>[4x]MSTLEQTIGNTPLVKLQRMGP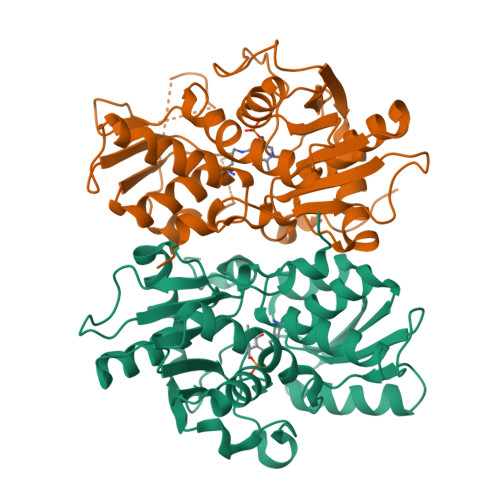DNGSEVWLKLEGNNPAGSVKDRAALSMIVEAEKRGRIKPGDVLIEATSGNTGIALAMIAALKGYRMKLLMPDNMSQERRAAMRAYGAELILVTKEQGMEGARDLALEMANRGEGKLLDQFNNPDNPKAHYTTTGPEIWQQTGGRITHFVSSMGTTGTITGVSEFMREQSKPVTIVGLQPEEGSSIPGIRRWPTEYLPGIFNASLVDEVLDIHQRDAENTMRELAVREGIFCGVSSGGAVAGALRVAKANPDAVVVAIICDRGDRYLSTGVFGEEHFSQGAGI> MQDAITAVINSSDVQGKYLDTAALEKLKSYFSTGELRVRAATTIAANAAAIVKEAVAKSLLYSDITRPGGNMYTTRRYAACIRD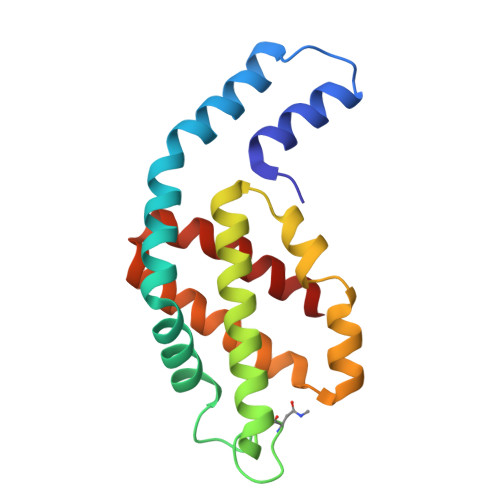LDYYLRYATYAMLAGDPSILDERVLNGLKETYNSLGVPISATVQAIQAMKEVTASLVGPDAGKEMGVYFDYICSGLS> MLKYKEILETIIEILKKNFTESIFIDDESVQGSEGSCFFVSILSVICTPVMLNTNNKDIVISIKYLPKPQSKSIRMYEISDELNKLFNRNIKVTDRKLNITKLEQSIKKEESIYVLNFTFTLNYLDSVYEEDVVYENMK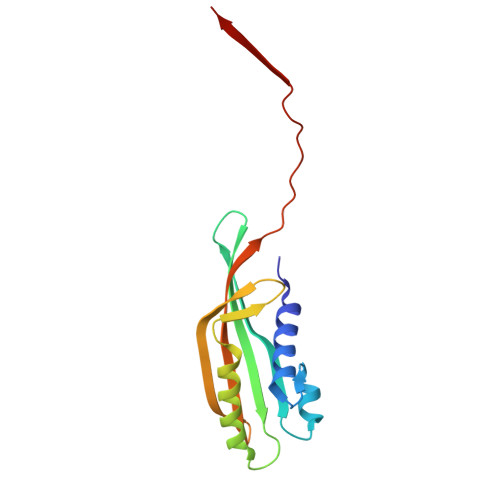EINLNLGE>[2x]KNNVPRLKLSYKEMLESNNVITFNGLANSSSYHTFLLDEERSRLYVGAKDHIFSFNLVNIKDFQKIVWPVSYTRRDECKWAGKDILKECANFIKVLEAYNQTHLYACGTGAFHPICTYIEVG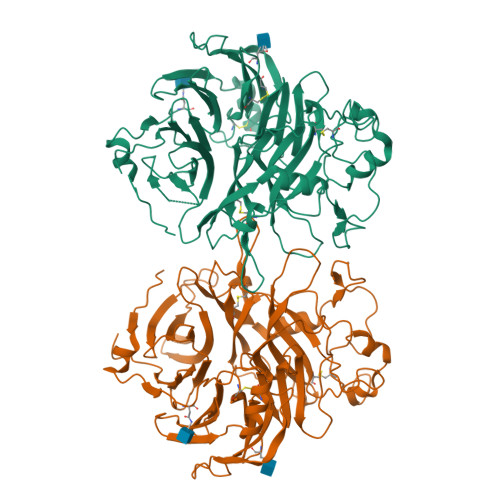HHPEDNIFKLQDSHFENGRGKSPYDPKLLTASLLIDGELYSGTAADFMGRDFAIFRTLGHHHPIRTEQHDSRWLNDPRFISAHLIPESDNPEDDKVYFFFRENAIDGEHSGKATHARIGQICKNDFGGHRSLVNKWTTFLKARLICSVPGPNGIDTHFDELQDVFLMNSKDPKNPIVYGVFTTSSNIFKGSAVCMYSMSDVRRVFLGPYAHRDGPNYQWVPYQGRVPYPRPGTCPSKTFGGFDSTKDLPDDVITFARSHPAMYNPVFPINNRPIMIKTDVNYQFTQIVVDRVDAEDGQYDVMFIGTDVGTVLKVVSVPKETWHDLEEVLLEEMTVFREPTTISAMELSTKQQQLYIGSTAGVAQLPLHRCDIY3-CHLOROPHENOL 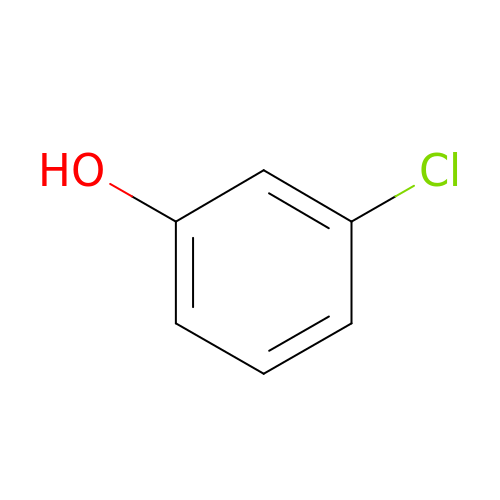| C6 H5 Cl O | HORNXRXVQWOLPJ-UHFFFAOYSA-N> GLSAVSKVERLMNLVIALLSTRTYLPAEKIRTTVAGYADSPSDEAFSRMFERDKNELRDLGIPLETGRVSKWDSTEGYRINRDSYALPPIGLTADEAAAVAVA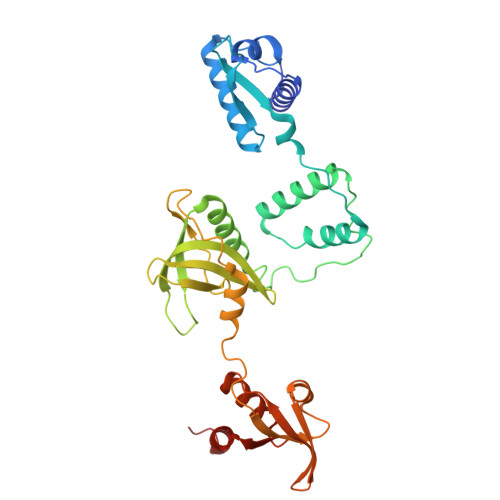TQLWQSPELVTATQNAVLKLRAAGVDVDADGVGVAIASTATLPGVRGSEEVLQSLLSAIDEGRAVQFEHRPSRSADYTTRTVEPWGVVTHRGRWYLVGHDRDREDTRTFRLSRISAAARPIGPAGAVQKPQDVNLRDIVRRAVAEQPTGERARIWIAGGRATALRRQAVTSTPRTIGGRAGEEITVDIGTWDRLAREIASYGSDAVALEPSSLRDDVVERLRAHAAGGER> SNAPTLGERLDSLHEIK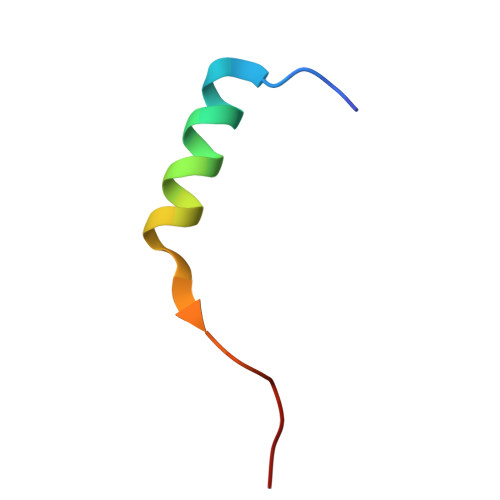SARRMDHFNDD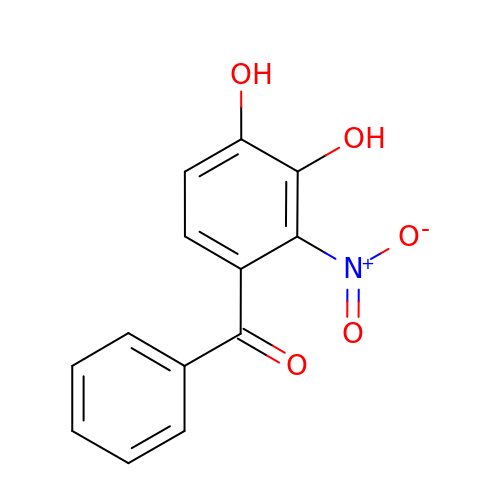(3,4-DIHYDROXY-2-NITROPHENYL)(PHENYL)METHANONE | C13 H9 N O5 | ICLKAUQIPVFHOI-UHFFFAOYSA-N> GAMLRVAVPNKGALSEPATEILAEAGYRRRTDSKDLTVIDPVNNVEFFFLRPKDIAIYVGSGELDFGITGRDLVCDSGAQVRERLALGFGSSSFRYAAPAGRNWTTADLAGMRIATAYPNLVRKDLATKGIEATVIRLDGAVEISVQLGVADAIADVVGSGRTLSQHDLVAFGEPLCDSEAV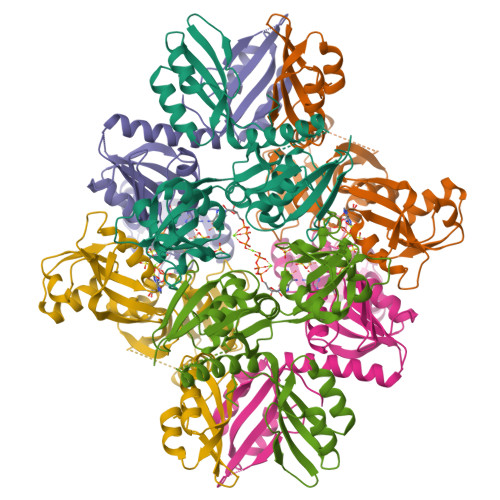LIERAGTDGQDQTEARDQLVARVQGVVFGQQYLMLDYDCPRSALKKATAITPGLESPTIAPLADPDWVAIRALVPRRDVNGIMDELAAIGAKAILASDIRFCRF> MKVVVIDAGHGAKDSGAVGISRKNYEKTFNLAMALKVESILKQNPKLEVVLTRSDDTFLELKQRVKVAENLKANVFVSIHANSSGSSASNGTETYYQRSASKAFANVMHKYFAP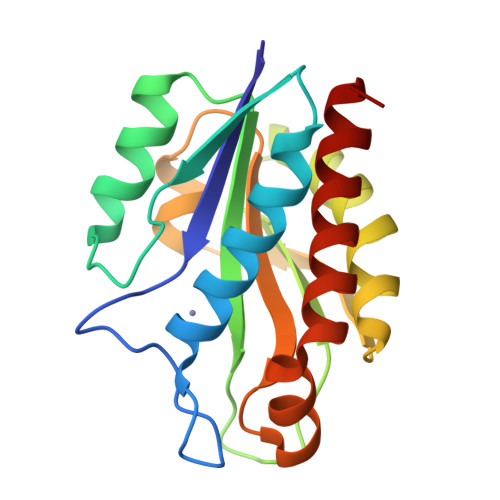ATGLTDRGIRYGNFHVIRETTMPAVLLEVGYLSNAKEEATLFDEDFQNRVAQGIADGITEYLDVK>[2x]MIAPLLKTLPFLAAAYAAELDLPNFSALNRRQDNSTSSSAGCSLDQTVAPGNLTLCGNATLFTTFRPKARFIAPEGWMNDPMGLYQRADGSIHAGYQSHPKHIQWGNISQGAAYSSDFTSWTDFNGSEGYKTIWPSQIYDIRGVFDGSIIKEGIDGYPTILYTSTSFGPLGATLNEAEGTETQSLAYTTDDGASWIKLGYGAGQNPVIYEW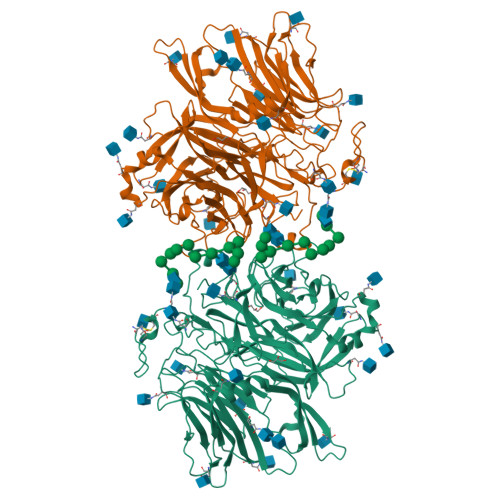PETNLTGFRDPYVFQSPRLEALLANTTSITNATGDHFATISGGVHGDGARLFLYRQHTTGEFIKWTYLGPLVTTGYKESYGEWSGNYGINFETAGVTRLNPAGAAWDNGSDTTAVDFVTFGTEQGRADHQNHWPLWAAVDYEVRDNGSIEAVIAYSGVQDWGRSYAYASFPVEGYRQVSVGWIYEDDDNVILAKQFGYQGAFTLFRDLFVKVVENVSPSTPGLFEQASWSTKNSTDGMSVTVTTLGQRVVPETLAAYKGNSTVSTLAPVMLNESAAAYTPFSSQPTDRFYALTGSFEFGLNTTAKAGFRVLASEEEYTDIWFDPASENLTVVRTASSLIKSFGNDTELAKVKLYEIVGAESKTLNLTVFVDGSVIEIYANDEVALSTRAYPWLANSTGAGLLADGTTAGDVVGVSGLELWDGLVDAWPARPANTSQGLVWDGPTAAMYGLFAGY>[2x]MELRVGNRYRLGRKIGSGSFGDIYLGTDIAAGEEVAIKLECVKTKHPQLHIESKIYKMMQGGVGIPTIRWCGAEGDYNVMVMELLGPSLEDLFNFCSRKFSLKTVLLLADQMISRIEYIHSKNFIHRDVKPDNFLMGLGKKG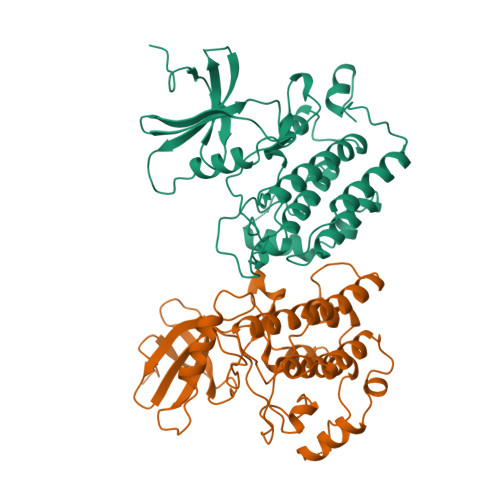NLVYIIDFGLAKKYRDARTHQHIPYRENKNLTGTARYASINTHLGIEQSRRDDLESLGYVLMYFNLGSLPWQGLKAATKRQKYERISEKKMSTPIEVLCKGYPSEFATYLNFCRSLRFDDKPDYSYLRQLFRNLFHRQGFSYDYVFDWNMLKFGASRAADDAERERRDREERLRH> MGSHQMKSEEHANMQLQQQAVLGLNWMQDSGEYKALAYQAYNAAKVAFDHAKVAKGKKKAVVANLDETMLDNSPYAGWQVQNNKPFDGKDWTRWVDARQSRAVPGAVEFNNYVNSHNGKVFYVTNRKDSTEKSGTIDDMKRLGFNGVEESAFYLKKDKSAKAARFAEIEKQGYEIVLYVGDNLDDFGNTVYGKLNADRRAFVDQNQGKFGKTFIMLPNANYGGWEGGLAEGYFKKDTQGQ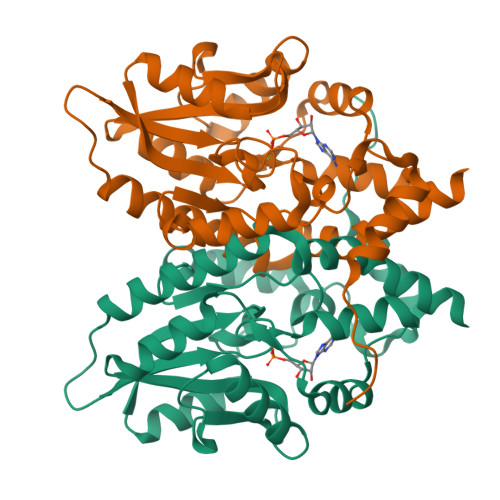IKARLDAVQAWDGKLEHHHHHH> GPHMGAKWHLGIRSQSRPNDIMAEVCRAIKQLDYEWKVVNPYYLRVRRKNPVTSTFSKMSLQLYQVDSRTYLLDFRSIDDGGGGGGGSHTIEFFEMCANLIKILAQ;> MFKAPPILPPHLLQVILNKDTGISCDPALLPEPNHVMLNHLYALSIKDGVMVLSATHRYKKKYVTTLLYKPI;> MESVAAESAPAPENEHSQETPESNSSVYTTFMKSHRCYDLIPTSSKLVV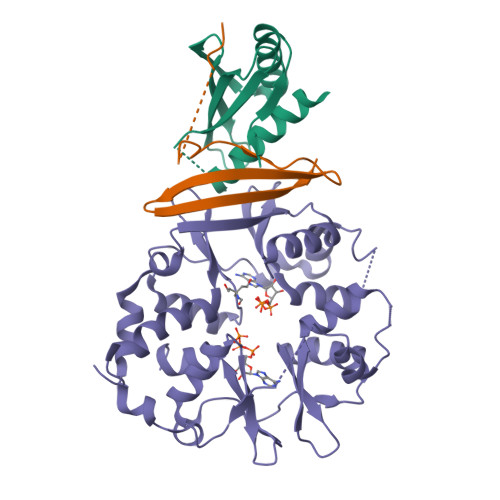FDTSLQVKKAFFALVTNGVRAAPLWDSKKQSFVGMLTITDFINILHRYYKSALVQIYELEEHKIETWREVYLQDSFKPLVCISPNASLFDAVSSLIRNKIHRLPVIDPESGNTLYILTHKRILKFLKLFITEFPKPEFMSKSLEELQIGTYANIAMVRTTTPVYVALGIFVQHRVSALPVVDEKGRVVDIYSKFDVINLAAEKTYNNLDVSVTKALQHRSHYFEGVLKCYLHETLEAIINRLVEAEVHRLVVVDEHDVVKGIVSLSDILQALVLTGGEKKP> MGHHHHHHVVPKTATSTETKTITRIIHYVDKVTNQNVKEDVVQPVTLSRTKTENKVTGVVTYGEWTTGNWDEVISGKIDKYKDPDIPTVESQEVTSDS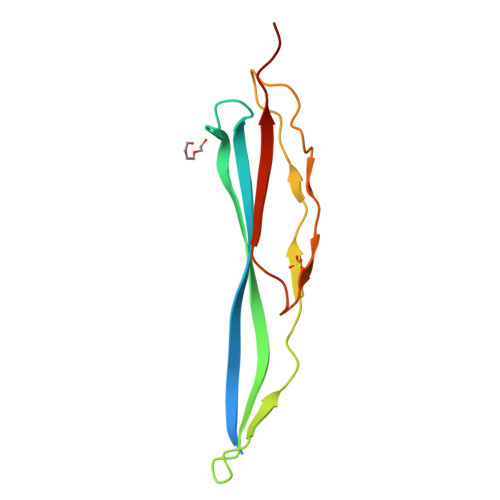SDKEITVRYDRLST>[2x]ATADAAAFPDLHRAAKL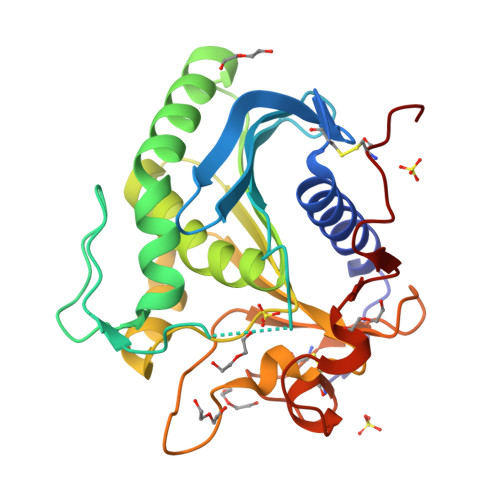SSAAYTGCIGKAFDVTIVKRIYDLVTDTNGFVGYSTEKKTIAVIMRGSTTITDFVNDIDIALITPELSGVTFPSDVKIMRGVHRPWSAVHDTIITEVKALIAKYPDYTLEAVGHSLGGALTSIAHVALAQNFPDKSLVSNALNAFPIGNQAWADFGTAQAGTFNRGNNVLDGVPNMYSSPLVNFKHYGTEYYSSGTEASTVKCEGQRDKSCSAGNGMYAVTPGHIASFGVVMLTAGCGYLS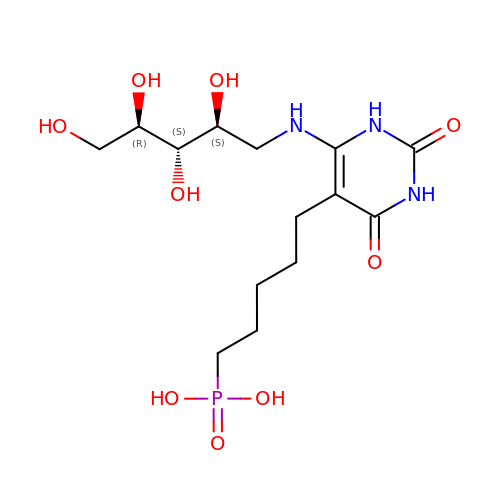5-(6-D-RIBITYLAMINO-2,4(1H,3H)PYRIMIDINEDIONE-5-YL) PENTYL-1-PHOSPHONIC ACID | C14 H26 N3 O9 P | BMATWAHJJFXMFA-AXFHLTTASA-N> MNQVAPFYADHVGSILRTKGIKDAREKFQSGEITALEL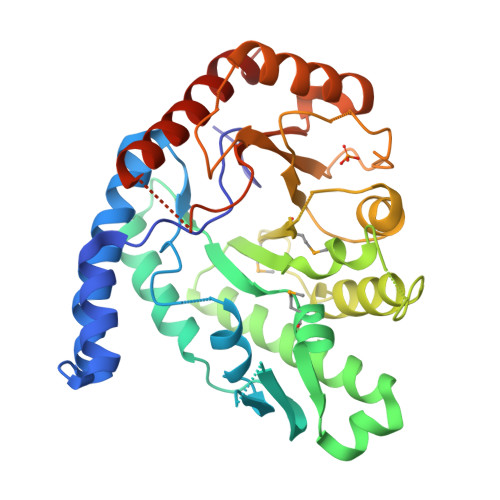RKIENTEIKYIVEKQKEVGLKSITDGEFRRAWWHFDFLENLDGVEGYDAAGGIQFSKVQTKSHSVKITGPIDFTTHPFIEDFIFLKEAVGDNHVAKQTIPSPAMLHYRGDIEYQPYLDDAEKFANDLATAYQKAIQAFYDAGCRYLQLDDTSWSYLCSDEQREVVRQRGFDPETLQETYKNLINEAIKHKPADMVITMHICRGNFRSTWIAEGGYGPVAETLFGKLNIDGFFLEYDNERSGDFAPLKYVTRPDLKIVLGLITSKTGELEDEAAIKARIEEASEIVPLSQLRLSPQCGFASTEEGNILTEEEQWDKLRYVVRLANDIWGELEHHHHHH>ASPNSPKDNTWIQAASLTWLMDMSSLLYQLISTRIPSFASPNGLHMREQTIDSNTGQIQIDNEHRLLRWDRRPPNDIFLNGFIPRVTNQNLSPVEDTHLLNYLRTNSPSIFVSTTRARYNNLGLEITPWTPHSANNNIIYRYEIFAPGGIDINASFSRNHNPFPNEDEITFPGGIRPEFIRSTYEYHNGEIVRIWINPNFINPSTLNDVSGPSNISKVFWHENHSEGNNMDSKGFILDLDYNQDFDMFAPNGEIPNNNLLNNNSLNVIQNSEYQIKNKKDRNIVVTLDSDYGGSPVESYKNFGFENQKWNIKYDSKKNAYKIYNRETPTLLLSWNSNSSNGEQVIRGYTESGSNNQYWTIEKNVNGFYKFRNLSDPSKILDLKDGNTLNKTPLVVSSENSSSSQEWLIEKTNYQTVKDGTYQVSSKLNENKVIEQISTNKVHIFSNSDKENQVWNLIYNPILKAYKIKSLKYPNYSLAWDSNNTRTIVAATGDYNDQYWLIERNEDNTYIIRNYENRKIVLDLSNGSTTDGNGLLGFEFHGGINQRWIIKPFSFNSIQDGIYQFMTVINQDLIADLTTNNYTIATK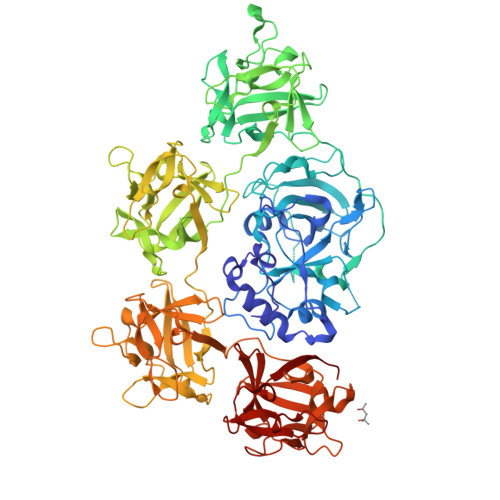TNNYSSNQKWTVTYNDKKRAYKIRNLQHAHLSLAWDSNHSDKIFGATGDYDDQYWIPILQTDGSFIFRNYKNPNKIFGTNGQPINDIPLKAQDVTGQNNQKWYLRHLNSSNNFTGYFNISSKKNFNKIITMNSNKTQAVIFDNIGINNQSWKLKYNDNKNAYQIHILDNFLYFQGGHNIVATMRNVTNDDLRSYWYVEYNFNKDGFIIRNAFDTSYVLDVFQGNFANNTPIITYQNYLNDNQLWNFIPSLGVEPR[2x]> DVSGTVCLSALPPEATDTLNLIASDGPFPYSQDGVVFQNRESVLPTQSYGYYHEYTVITPGAR;> TRGTRRIITGEATQEDYY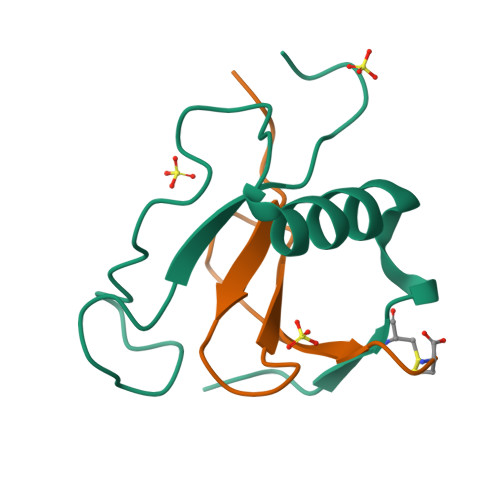TGDHYATFSLIDKTC(3S)-3-(5-azanyl-2-methyl-4-oxidanylidene-quinazolin-3-yl)piperidine-2,6-dione 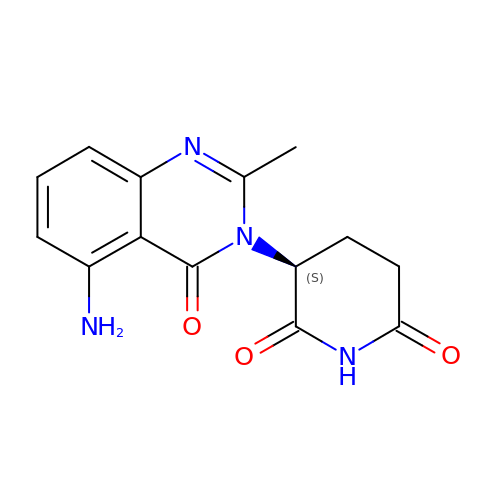| C14 H14 N4 O3 | RSNPAKAFCAAMBH-JTQLQIEISA-N> MQLF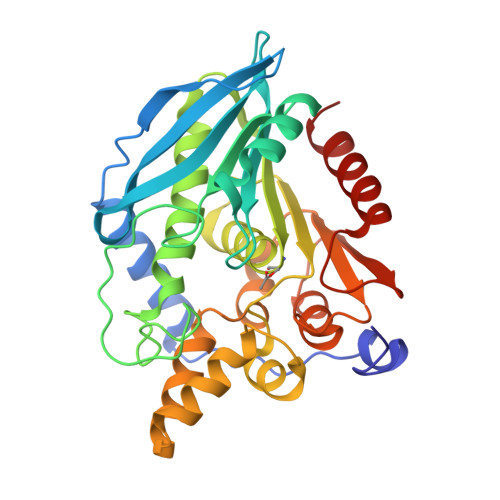DLSLEELKKYKPKKTARPDFSDFWKKSLEELRQVEAEPTLESYDYPVKGVKVYRLTYQSFGHSKIEGFYAVPDQTGPHPALVRFHGYNASYDGGIHDIVNWALHGYATFGMLVRGQGGSEDTSVTPGGHALGWMTKGILSKDTYYYRGVYLDAVRALEVIQSFPEVDEHRIGVIGGSQGGALAIAAAALSDIPKVVVADYPYLSNFERAVDVALEQPYLEINSYFRRNSDPKVEEKAFETLSYFDLINLAGWVKQPTLMAIGLIDKITPPSTVFAAYNHLETDKDLKVYRYFGHEFIPAFQTEKLSFLQKHLLLST> ETGGSWAQVKLLESGGKVTHEGQSVTLTCKASGFNFKDYAMSWHWNPSGSNRQFVASISPKTGSKREYKPSIQGRALITRNNEANTVSLTLRQLRKEDSGIYYCAKPSGLRQWGPKWEPLAEQWENFGPGTELTVLPLEKTLLTESGGGTYQAGKTLSLKCQTSGFQFKTSQLDWYLWTPGHAPLWLTGLNSSSTDATEGRITSSREDNKNQIFLQIEDLGLRDSGQYHCARRVGNGDDTDKLVFGL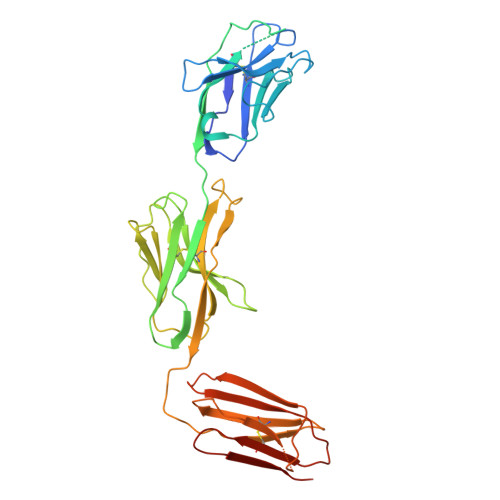GTRVIVEPRPAAPLSPSVFLVRDQDAVACLIRNFYPKELHVSLTSSGTLISAQSLSLAPTASGTYSAIHIGRVGENDAITCSVKHLGKEIHMSHQAGSLVPR> XXXXXXXXXXXXXXXXXXXXXXXXXXXXXXXXXXXXXXXXXXXXXXXXXXXXXXXXXXXXXXXXXXXXXXXXXXXXXXXXXXXXXXXXXXXXXXXXXXXXXXXXXXXXXXXXXXXXXXXXXXXXXXXXXXXXXXXXXXXXXXXXXXXXXXXXXXXXXXXXXXXXXXXXXXXXXXXXXXXXXXXXXXXXXXPSVPECFTIEKKSSYFIIEPQDLSTKVASICGVIVPKVHTIHDKVFYPLTFVPTHKTVSSLRQLGRKIQNSTPIMLIGKAGSGKTFLINELSKYMGCHDSIVKIHLGEQTDAKLLIGTYTSGDKPGTFEWRAGVLATAVKEGRWVLIEDIDKAPTDVLSILLSLLEKRELTIPSRGETVKAANGFQLISTVRINEDHQKDSSNKIYNLNMIGMRIWNVIELEEPSEEDLTHILAQKFPILTNLIPKLIDSYKNVKSIYMNTKFISLNKGAHTRVVSVRDLIKLCERLDILFKNNGINKPDQLIQSSVYDSIFSEAADCFAGAIGEFKALEPIIQAIGESLDIASSRISLFLTQHVPTLENLDDSIKIGRAVLLKEKLNIQKKSMNSTLFAFTNHSLRLMEQISVCIQMTEPVLLVGETGTGKTTVVQQLAKMLAKKLTVINVSQQTETGDLLGGYKPVNSKTVAVPIQENFETLFNATFSLKKNEKFHKMLHRCFNKNQWKNVVKLWNEAYKMAQSILKITNTENENENAKKKKRRLNTHEKKLLLDKWADFNDSVKKFEAQSSSIENSFVFNFVEGSLVKTIRAGEWLLLDEVNLATADTLESISDLLTEPDSRSILLSEKGDAEPIKAHPDFRIFACMNPATDVGKRDLPMGIRSRFTEIYVHSPERDITDLLSIIDKYIGKYSVSDEWVGNDIAELYLEAKKLSDNNTIVDGSNQKPHFSIRTLTRTLLYVTDIIHIYGLRRSLYDGFCMSFLTLLDQKSEAILKPVIEKFTLGRLKNVKSIMSQTPPSPGPDYVQFKHYWMKKGPNTIQEQAHYIITPFVEKNMMNLVRATSGKRFPVLIQGPTSSGKTSMIKYLADITGHKFVRINNHEHTDLQEYLGTYVTDDTGKLSFKEGVLVEALRKGYWIVLDELNLAPTDVLEALNRLLDDNRELFIPETQEVVHPHPDFLLFATQNPPGIYGGRKILSRAFRNRFLELHFDDIPQDELEIILRERCQIAPSYAKKIVEVYRQLSIERSASRLFEQKNSFATLRDLFRWALRDAVGYEQLAASGYMLLAERCRTPQEKVTVKKTLEKVMKVKLDMDQYYASLEDKSLEAIGSVTWTKGMRRLSVLVSSCLKNKEPVLLVGETGCGKTTICQLLAQFMGRELITLNAHQNTETGDILGAQRPVRNRSEIQYKLIKSLKTALNIANDQDVDLKELLQLYSKSDNKNIAEDVQLEIQKLRDSLNVLFEWSDGPLIQAMRTGNFFLLDEISLADDSVLERLNSVLEPERSLLLAEQGSSDSLVTASENFQFFATMNPGGDYGKKELSPALRNRFTEIWVPSMEDFNDVNMIVSSRLLEDLKDLANPIVKFSEWFGKKLGGGNATSGVISLRDILAWVEFINKVFPKIQNKSTALIQGASMVFIDALGTNNTAYLAENENDLKSLRTECIIQLLKLCGDDLELQQIETNEIIVTQDELQVGMFKIPRFPDAQSSSFNLTAPTTASNLVRVVRAMQVHKPILLEGSPGVGKTSLITALANITGNKLTRINLSEQTDLVDLFGADAPGERSGEFLWHDAPFLRAMKKGEWVLLDEMNLASQSVLEGLNACLDHRGEAYIPELDISFSCHPNFLVFAAQNPQYQGGGRKGLPKSFVNRFSVVFIDMLTSDDLLLIAKHLYPSIEPDIIAKMIKLMSTLEDQVCKRKLWGNSGSPWEFNLRDTLRWLKLLNQYSICEDVDVFDFVDIIVKQRFRTISDKNKAQLLIEDIFGKFSTKENFFKLTEDYVQINNEVALRNPHYRYPITQNLFPLECNVAVYESVLKAINNNWPLVLVGPSNSGKTETIRFLASILGPRVDVFSMNSDIDSMDILGGYEQVDLTRQISYITEELTNIVREIISMNMKLSPNATAIMEGLNLLKYLLNNIVTPEKFQDFRNRFNRFFSHLEGHPLLKTMSMNIEKMTEIITKEASVKFEWFDGMLVKAVEKGHWLILDNANLCSPSVLDRLNSLLEIDGSLLINECSQEDGQPRVLKPHPNFRLFLTMDPKYGELSRAMRNRGVEIYIDELHSRSTAFDRLTLGFELGENIDFVSIDDGIKKIKLNEPDMSIPLKHYVPSYLSRPCIFAQVHDILLLSDEEPIEESLAAVIPISHLGEVGKWANNVLNCTEYSEKKIAERLYVFITFLTDMGVLEKINNLYKPANLKFQKALGLHDKQLTEETVSLTLNEYVLPTVSKYSDKIKSPESLYLLSSLRLLLNSLNALKLINEKSTHGKIDELTYIELSAAAFNGRHLKNIPRIPIFCILYNILTVMSENLKTESLFCGSNQYQYYWDLLVIVIAALETAVTKDEARLRVYKELIDSWIASVKSKSDIEITPFLNINLEFTDVLQLSRGHSITLLWDIFRKNYPTTSNSWLAFEKLINLSEKFDKVRLLQFSESYNSIKDLMDVFRLLNDDVLNNKLSEFNLLLSKLEDGINELELISNKFLNKRKHYFADEFDNLIRYTFSVDTAELIKELAPASSLATQKLTKLITNKYNYPPIFDVLWTEKNAKLTSFTSTIFSSQFLEDVVRKSNNLKSFSGNQIKQSISDAELLLSSTIKCSPNLLKSQMEYYKNMLLSWLRKVIDIHVGGDCLKLTLKELCSLIEEKTASETRVTFAEYIFPALDLAESSKSLEELGEAWITFGTGLLLLFVPDSPYDPAIHDYVLYDLFLKTKTFSQNLMKSWRNVRKVISGDEEIFTEKLINTISDDDAPQSPRVYRTGMSIDSLFDEWMAFLSSTMSSRQIKELVSSYKCNSDQSDRRLEMLQQNSAHFLNRLESGYSKFADLNDILAGYIYSINFGFDLLKLQKSKDRASFQISPLWSMDPINISCAENVLSAYHELSRFFKKGDMEDTSIEKVLMYFLTLFKFHKRDTNLLEIFEAALYTLYSRWSVRRFRQEQEENEKSNMFKFNDNSDDYEADFRKLFPDYEDTALVTNEKDISSPENLDDIYFKLADTYISVFDKDHDANFSSELKSGAIITTILSEDLKNTRIEELKSGSLSAVINTLDAETQSFKNTEVFGNIDFYHDFSIPEFQKAGDIIETVLKSVLKLLKQWPEHATLKELYRVSQEFLNYPIKTPLARQLQKIEQIYTYLAEWEKYASSEVSLNNTVKLITDLIVSWRKLELRTWKGLFNSEDAKTRKSIGKWWFYLYESIVISNFVSEKKETAPNATLLVSSLNLFFSKSTLGEFNARLDLVKAFYKHIQLIGLRSSKIAGLLHNTIKFYYQFKPLIDERITNGKKSLEKEIDDIILLASWKDVNVDALKQSSRKSHNNLYKIVRKYRDLLNGDAKTIIEAGLLYSNENKLKLPTLKQHFYEDPNLEASKNLVKEISTWSMRAAPLRNIDTVASNMDSYLEKISSQEFPNFADLASDFYAEAERLRKETPNVYTKENKKRLAYLKTQKSKLLGDALKELRRIGLKVNFREDIQKVQSSTTTILANIAPFNNEYLNSSDAFFFKILDLLPKLRSAASNPSDDIPVAAIERGMALAQSLMFSLITVRHPLSEFTNDYCKINGMMLDLEHFTCLKGDIVHSSLKANVDNVRLFEKWLPSLLDYAAQTLSVISKYSATSEQQKILLDAKSTLSSFFVHFNSSRIFDSSFIESYSRFELFINELLKKLENAKETGNAFVFDIIIEWIKANKGGPIKKEQKRGPSVEDVEQAFRRTFTSIILSFQKVIGDGIESISETDDNWLSASFKKVMVNVKLLRSSVVSKNIETALSLLKDFDFTTTESIYVKSVISFTLPVITRYYNAMTVVLERSRIYYTNTSRGMYILSTILHSLAKNGFCSPQPPSEEVDDKNLQEGTGLGDGEGAQNNNKDVEQDEDLTEDAQNENKEQQDKDERDDENEDDAVEMEGDMAGELEDLSNGEENDDEDTDSEEEELDEEIDDLNEDDPNAIDDKMWDDKASDNSKEKDTDQNLDGKNQEEDVQAAENDEQQRDNKEGGDEDPNAPEDGDEEIENDENAEEENDVGEQEDEVKDEEGEDLEANVPEIETLDLPEDMNLDSEHEESDEDVDMSDGMPDDLNKEEVGNEDEEVKQESGIESDNENDEPGPEEDAGETETALDEEEGAEEDVDMTNDEGKEDEENGPEEQAMSDEEELKQDAAMEENKEKGGEQNTEGLDGVEEKADTEDIDQEAAVQQDSGSKGAGADATDTQEQDDVGGSGTTQNTYEEDQEDVTKNNEESREEATAALKQLGDSMKEYHRRRQDIKEAQTNGEEDENLEKNNERPDEFEHVEGANTETDTQALGSATQDQLQTIDEDMAIDDDREEQEVDQKELVEDADDEKMDIDEEEMLSDIDAHDANNDVDSKKSGFIGKRKSEEDFENELSNEHFSADQEDDSEIQSLIENIEDNPPDASASLTPERSLEESRELWHKSEISTADLVSRLGEQLRLILEPTLATKLKGDYKTGKRLNMKRIIPYIASQFRKDKIWLRRTKPSKRQYQIMIALDDSKSMSESKCVKLAFDSLCLVSKTLTQLEAGGLSIVKFGENIKEVHSFDQQFSNESGARAFQWFGFQETKTDVKKLVAESTKIFERARAMVHNDQWQLEIVISDGICEDHETIQKLVRRARENKIMLVFVIIDGITSNESILDMSQVNYIPDQYGNPQLKITKYLDTFPFEFYVVVHDISELPEMLSLILRQYFTDLASS

The AAA+ (ATPases Associated with various cellular Activities) family member Rea1 (or Midasin) consists of nearly 5000 amino acids and generates force to mechanically remove assembly factors. Rea1 consists of an N-terminal α-helical domain (NTD), a ring of six AAA+ domains, and the C-terminal tail. The Rea1 tail is subdivided into an α-helical linker region, a D/E-rich region, and a MIDAS (Metal-Ion-Dependent Adhesion Site) domain which is responsible for the interaction with the Ytm1 and Rsa4 substrates. Rea1 pulls out the Ytm1 complex to promote the transfer of pre-60S particles from the nucleolus to the nucleoplasm.

To provide insights into these open questions, we have determined the S. cerevisiae Rea1 structure in complex with ADP by CryoEM, which revealed the NTD, the AAA+ ring, as well as the linker part of the Rea1 tail. Focused refinement of the NTD-AAA+ ring area and the linker resulted in two cryoEM maps with resolutions of 4.4 Å and 3.9 Å, respectively. In the NTD-AAA+ ring map, the main-chain is well-resolved in the NTD, AAA1, AAA2, as well as AAA6, and side-chains are occasionally visible. The AAA3-AAA5 part of the AAA +ring is more flexible, but still allowed docking of AAA+ domains into the map. In the structure presented here, the nucleotide binding sites of AAA1 and AAA6 are closed and show densities consistent with a bound nucleotide. We interpreted this bound nucleotide as ADP as there is not enough density to fit a γ-phosphate. In contrast to the AAA1 and AAA6 sites, the AAA2 and AAA5 nucleotide-binding sites of the Rea1 AAA+ ring are wide open as indicated by large gaps between modules AAA2/AAA3 and AAA5/AAA6. The open state of the latter sites is stabilised by the AAA2L-H2α insert which sits in the AAA+ ring centre. The β-sheet base of AAA2L-H2α is interacting with the AAA1L H2-β-sheet and the α-helices of AAA2L-H2α contact the tips of the AAA3L and AAA5L H2-β-sheets to prevent the closure of the AAA2 and AAA5 sites. Our structural analysis suggests that the AAA2L-H2α insert impairs the hydrolytic activity of all functional Rea1 nucleotide binding sites.>SVLFVDSFDGSSVVPDTAVWKLCTYANNAWSQWFRDVNGYENVKVEDGYLKLRACKDNGTYKNGGVFSKIGFPCGTRLEVKARLTKLVRGGFPAIWQMPIGAPEWPRGGEIDLMEWVQGTPLQIYQTVHTYYINGANGSAGVTNKNPDKNFDVTKDHVY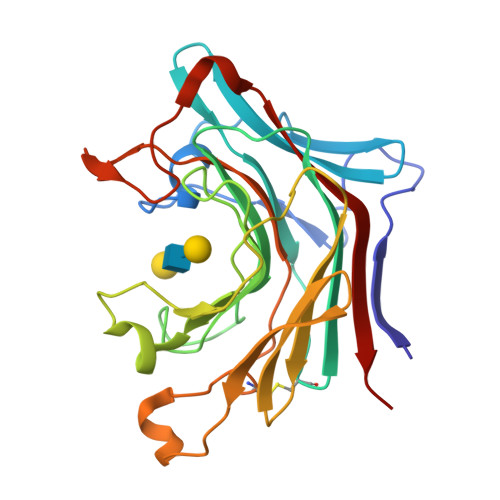AVERTEKEVIFYVDGKETWRYGNQYLDEGKLQYPFCEYPFNIILNFSLGGELNGRMTWSGEICDEDLPGEMWVDWVRVVSLN[3x]>MAEQVLPQALYLSNMRKAVKIRERTPEDIFKPTNGIIHHFKTMHRYTLEMFRTCQFCPQFREIIHKALIDRNIQATLESQKKLNWCREVRKLVALKTNGDGNCLMHATSQYMWSVQDTDLVLRKALFSTLKETDTRNFKFRWQLESLKSQEFVETGLCYDTRNWNDEWDNLIKMASTDTPMARSGLQYNSLEEIHIFVLCNILRRPIIVISDKMLRSLESGSNFAPLKVGGIYLPLHWPAQECYRYPIVLGYDSHHFVPLVTLKDSGPEIRAVPLVNRDRGRFEDLKVHFLTDPENEMKEKLLKEYLMVIEIPVQ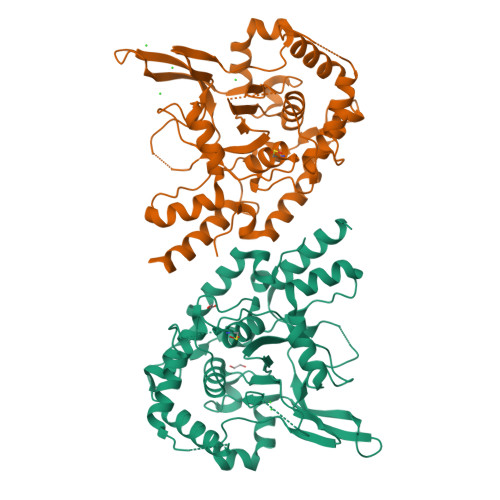GWDHGTTHLINAAKLDEANLPKEINLVDDYFELVQHEYKKWQENSEQGRRE[2x]>[2x]GIDPFTKMTRPSSDLTAFREHFAKAKHIAIITGAGVSAESGVPTFRGPGGFWRKWQAQDLATPEAFSRDPSLVWEFYHYRREVMRSKMPNPAHLAIAECEARLGQQGRS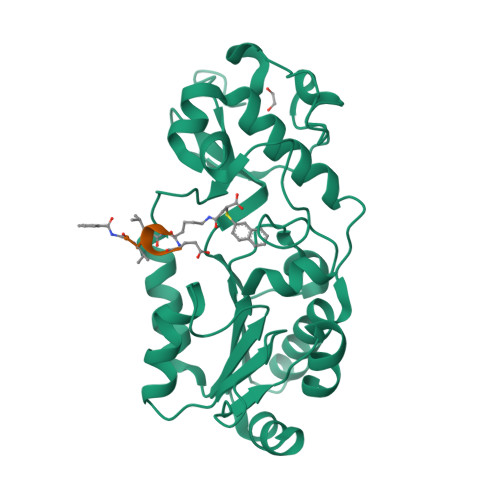VVIITQNIDELHHRAGSKHVYEIHGSLFKTRCMSCGEVKANHKSPICPALDGKGAPDPNTKEARIPVELLPRCERKSCNGLLRPHVVWFGETLDSDILTAVERELEKCDLCLVVGTSSIVYPAAMFAPQVASRGVPVAEFNMECTPATQRFKYHFEGPCGSTLPPALERHESEAV> GSSHHHHHHSGDPASMIINNRNESQPRRVVVTGLGVVAPTGVGVNEFWNNIHNGKSGVSKYEWGRERFGFKSGAIGQVYG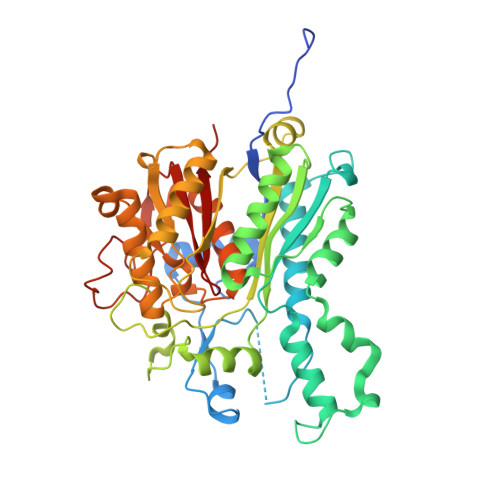SDGNNKEFVLKSERKYLQFALDAAEMAMQDANLRPSDIDGRRFGVAIATAIADAAGMEECLLRITKGGKENIHPDLIKSEDYDSFDFSSAATSVAKKYGASMSVSNISTGCAAGLDALGIAMEHIRYGRADIMLAGASEAPLCPLSIGSFEALGALSSRELENQQAATCPFSLERDGFVIAEGCGILILESYEHAKQRGAHIYAELAGYASVNNAYHMTDLPADGMAMARCIDMALKDAQISPSTVNYISAHGSSTAQNDINESNAIKFVLGESAFGIPINSLKSMTGHALAAANAIESVALCLEIEKQYVHPTINYQTPDPDCDLDYIPNQGCSYPIKTALKLSSGFSGIHSVIVMRAVDNA>[10x]MLFGRLTERAQRVLAHAQEEAIRLNHSNIGTEHLLLGLMKEPEGIAAKVLESFNITEDKVIEEVEKLIGHGQDHVGTLHYTPRAKKVIELSMDEARKLHHNFVGTEHILLGLIRENEGVAARVFANLDLNITKARAQVVKALGNPEMSNKNAQASKSNNTPTLDSLARDLTVIAKDGTLDPVIGRDKEITRVIEVLSRRTKNNPVLIGEPGVGKTAIAEGLAQAIVNNEVPETLKDKRVMSLDMGTVVAGTKYRGEFEERLKKVMEEIQQAGNVILFIDELHTLVGAGGAEGAIDASNILKPALARGELQCIGATTLDEYRKNIEKDAALERRFQPVQVDEPSVVDTVAILKGLRDRYEAHHRINISDEAIEAAVKLSNRYVSDRFLPDKAIDLIDEASSKVRLKSHTTPNNLKEIEQEIEKVKNEKDAAVHAQEFENAANLRDKQTKLEKQYEEAKNEWKNTQNGMSTSLSEEDIAEVIAGWTGIPLTKINETESEKLLSLEDTLHERVIGQKDAVNSISKAVRRARAGLKDPKRPIGSFIFLGPTGVGKTELARALAESMFGDDDAMIRVDMSEFMEKHAVSRLVGAPPGYVGHDDGGQLTEKVRRKPYSVILFDEIEKAHPDVFNILLQVLDDGHLTDTKGRTVDFRNTIIIMTSNVGAQELQDQRFAGFGGSSDGQDYETIRKTMLKELKNSFRPEFLNRVDDIIVFHKLTKEELKEIVTMMVNKLTNRLSEQNINIIVTDKAKDKIAEEGYDPEYGARPLIRAIQKTIEDNLSELILDGNQIEGKKVTVDHDGKEFKYDIAEQTSETKTPSQA

The bacterial AAA+ chaperone ClpC associates with the peptidase ClpP to form a central proteolytic machinery of Gram-positive bacteria. The ClpC-ClpP machinery acts in regulatory and general proteolysis, controlling multiple cellular pathways and differentiation processes and is crucial for bacterial stress resistance and virulence. ClpC activity crucially relies on cooperation with adaptor proteins including MecA, that target specific substrates while concurrently stimulating ClpC ATPase activity. Here, we report on an unexpected mode of AAA+ chaperone control involving transition between an inactive resting state and a functional hexamer as revealed by determining the cryoEM-structures of S. aureus ClpC in absence and presence of MecA.

The structure of ClpC on its own was solved at 8.4 Å resolution using ~90.000 collected particles. Surprisingly, raw images and subsequent 2D classification revealed immediately that ClpC assumes a conformation different from the canonical hexameric arrangement of AAA+ proteins (Figure 3—figure supplement 1A/B). Attempts of 3D classification and refinement using the existing ClpC-MecA structures failed to give a refined map, indicating that on its own, ClpC assumes a substantially different conformation. Indeed, reconstructions revealed that ClpC without MecA assembles into an oligomeric assembly made of two open spirals that interact via head-to-head contacts mainly mediated by the MDs (Figure 3A/B). Additionally, high-threshold noise on the open part of the spiral indicates higher dynamics of this region, suggesting exchange of subunits. Accordingly, for peripheral ClpC subunits there is not sufficient density to account for all ClpC domains. The AAA+ domains are staggered with a rise of ~20 Å per subunit. N-domains domains are packed between MDs and are displaced so that they lie on top of the adjacent small AAA1 subdomain (Figure 3B/C). The MDs coiled-coils constitute the backbone of the spiral and mediate the spiral head-to-head contacts, which involve residues F436, R443 and D444 providing a structural rationale for the activated states of respective MD mutants. We envision the helical ClpC assembly as a dynamic inactive resting state, which will interfere with substrate binding, association of the ClpP peptidase and interaction with adaptor proteins.>MSNVPHKSSLPEGIRPGTVLRIRGLVPPNASRFHVNLLCGEEQGSDAALHFNPRLDTSEVVFNSKEQGSWGREERGPGVPFQRGQPFEVLIIASDDGFKAVVGDAQYHHFRHRLPLARVRLVEVGGDV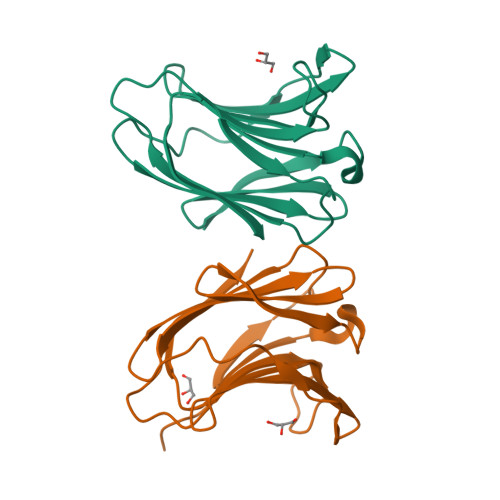QLDSVRIF[2x]The ABC transporter CydDC plays a central role in the biogenesis of membrane-integrated and soluble cytochromes. Here, we used cellular, biochemical, structural and computational methods to characterize the structure and function of the heterodimeric bacterial ABC transporter CydDC. We provide multi-level evidence that CydDC is a heme transporter required for functional maturation of cytochrome bd, a pharmaceutically relevant drug target. Each subunit is composed of a membrane domain formed by six transmembrane α-helices (TMH), an N-terminal cytoplasmic elbow helix oriented parallel to the membrane plane and a cytoplasmic NBD.

Of the two constructed Walker B variants, only CydDCE500Q could be isolated in sufficient yield, purity and stability. The nucleotide and substrate-free, inward-facing conformation of CydDC IFasisolatedapo, obtained in as isolated conditions, exhibits canonical features of type IV ABC transporters. In contrast to the turnover dataset of CydDCE500Q, biochemically defined CydDCE500Q cryo-EM samples revealed conformational heterogeneity reflected by structures of IFasisolatedapo, IFconfinedheme and Occreturnapo states.

> MRALLPYLALYKRHKWMLSLGIVLAIVTLLASIGLLTLSGWFLSASAVAGVAGLYSFNYMLPAAGVRGAAITRTAGRYFERLVSHDATFRVLQHLRIYTFSKLLPLSPAGLARYRQGELLNRVVADVDTLDHLYLRVISPLVGAFVVIMVVTIGLSFLDFTLAFTLGGIMLLTLFLMPPLFYRAGKSTGQNLTHLRGQYRQQLTAWLQGQAELTIFGASDRYRTQLENTEIQWLEAQRRQSELTALSQAIMLLIGALAVILMLWMASGGVGGNAQPGALIALFVFCALAAFEALAPVTGAFQHLGQVIASAVRISDLTDQKPEVTFPDTQTRVADRVSLTLRDVQFTYPEQSQQALKGISLQVNAGEHIAILGRTGCGKSTLLQQLTRAWDPQQGEILLNDSPIASLNEAALRQTISVVPQRVHLFSATLRDNLLLASPGSSDEALSEILRRVGLEKLLEDAGLNSWLGEGGRQLSGGELRRLAIARALLHDAPLVLLDQPTEGLDATTESQILELLAEMMREKTVLMVTHRLRGLSRFQQIIVMDNGQIIEQGTHAELLARQGRYYQFKQGL;> MNKSRQKELTRWLKQQSVISQRWLNISRLLGFVSGILIIAQAWFMARILQHMIMENIPREALLLPFTLLVLTFVLRAWVVWLRERVGYHAGQHIRFAIRRQVLDRLQQAGPAWIQGKPAGSWATLVLEQIDDMHDYYARYLPQMALAVSVPLLIVVAIFPSNWAAALILLGTAPLIPLFMALVGMGAADANRRNFLALARLSGHFLDRLRGMETLRIFGRGEAEIESIRSASEDFRQRTMEVLRLAFLSSGILEFFTSLSIALVAVYFGFSYLGELDFGHYDTGVTLAAGFLALILAPEFFQPLRDLGTFYHAKAQAVGAADSLKTFMETPLAHPQRGEAELASTDPVTIEAEELFITSPEGKTLAGPLNFTLPAGQRAVLVGRSGSGKSSLLNALSGFLSYQGSLRINGIELRDLSPESWRKHLSWVGQNPQLPAATLRDNVLLARPDASEQELQAALDNAWVSEFLPLLPQGVDTPVGDQAARLSVGQAQRVAVARALLNPCSLLLLDEPAASLDAHSEQRVMEALNAASLRQTTLMVTHQLEDLADWDVIWVMQDGRIIEQGRYAELSVAGGPFATLLAHRQEEI>MIQSQINRNIRLDLADAILLSKAKKDLSFAEIADGTGLAEAFVTAALLGQQALPADAARLV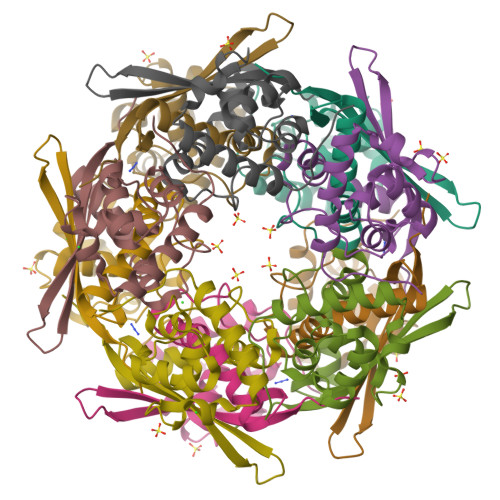GAKLDLDEDSILLLQMIPLRGCIDDRIPTDPTMYRFYEMLQVYGTTLKALVHEKFGDGIIAAINFKLDVKKVADPEGGERAVITLDGKYLPTKPF[10x]2-cyclopentyl-4-(5-phenyl-1H-pyrrolo[2,3-b]pyridin-3-yl)benzoic acid | C25 H22 N2 O2 | 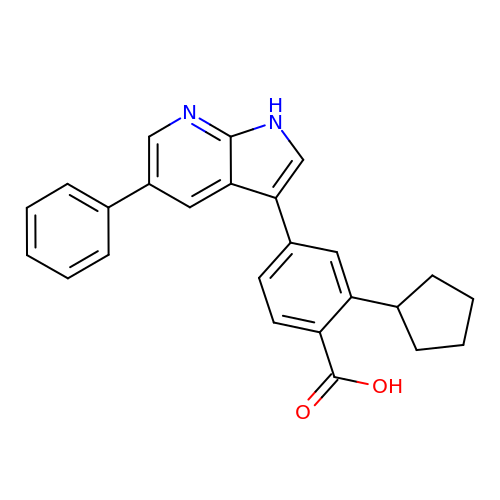WVSBGSNVCDAMCF-UHFFFAOYSA-N>[6x]AAASMDAVTAEKFSPASFLDKKETGVLHFVKYHGLGNDFILVDNRDSSEPKITQEQAAKLCDRNFGVGADGVIF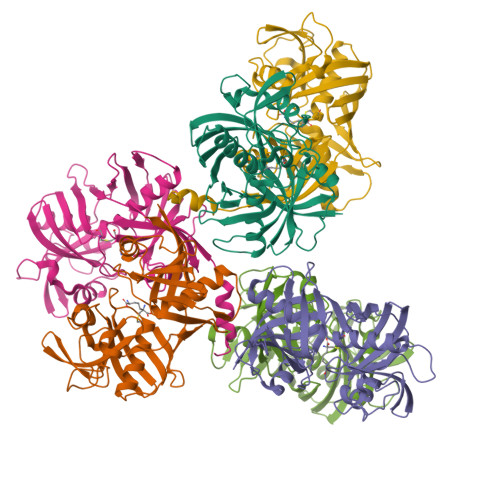AMPGVNGTDYAMRIFNSDGSEPEMCGNGVRCFARFIAELENLQGKHSFTIHTGAGLIVPEIQDDGQVKVDMGTPILKAQDVPTKLSGNKGEAVVEAELVVDGVSWNVTCVSMGNPHCITFGKKGGPNLKVDDLNLPEIGPKFEHHEMFPARTNTEFVEVLSRSHLKMRVWERGAGATLACGTGACALVVAAVLEGRADRKCTVDLPGGPLEIEWKQEDNHIYMTGPAEAVFYGSALLHHHHHH> GASPSAQELKEQGNRLFVGRKYPEAAACYGRAITRNPLVAVYYTNRALCYLKMQQHEQALADCRRALELDGQSVKAHFFLGQCQLEMESYD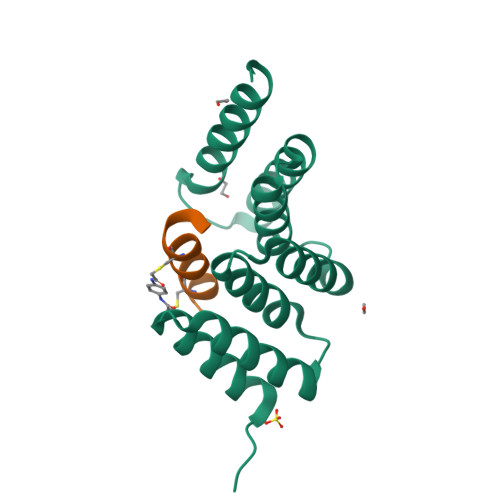EAIANLQRAYSLAKEQRLNFGDDIPSALRIAKKKRWNSIEERR;> XPWEDCAWFAWACYNIX>MVHFHPFGNVNFYEMDWSLKGDLWAHDPVIAKEGSRWYVFHTGSGIQIKTSEDGVHWENMGRVFPSLPDWCKQYVPEKDEDHLWAPDICFYNGIYYLYYSVSTFGKNTSVIGLATNRTLDPRDPDYEWKDMGPVIHSTASDNYNAINPNVVFDQEGQPWLSFGSFWSGIQLIQLDTETMKPAAQAELLTIASRGEEPNAIEAPFIVCRNGYYYLFVSFDFCCRGIESTYKIAVGRSKDITGPYVDKNGVSMMQGGGTILDAGNDRWIGPGHCAVYFSGVSAILVNHAYDALKNGEPTLQIRPLYWDDEGWPYLLEHHHHHH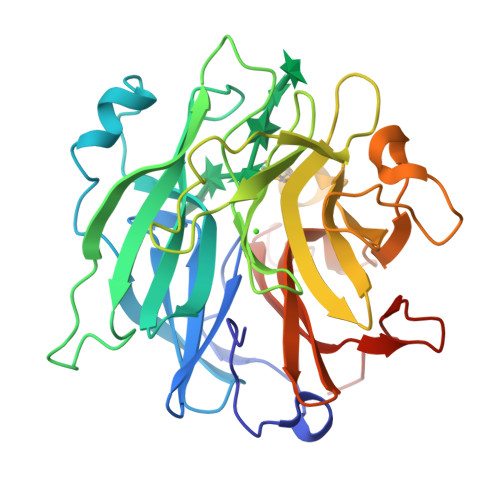[2x]>MKHHHHHHPMSDKIIHLTDDSFDTDVLKADGAILVDFWAEWCGPCKMIAPILDEIADEYQGKLTVAKLNIDQNPGTAPKYGIRGIPTLLLFKNGEVAATKVGALSKGQLKEFLDANLAGSAMESTVMVLRNMVDPKD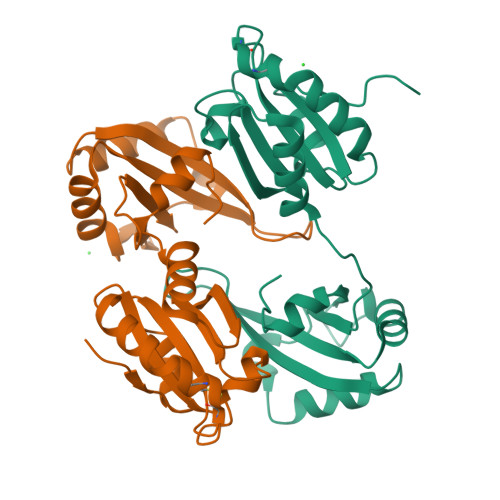IDDDLEGEVTEECGKFGAVNRVIIYQEKQGEEEDAEIIVKIFVEFSIASETHKAIQALNGRWFAGRKVVAEVYDQERFDNSDLSA[8x]> ELSTSLYKKAGFHHHHHHENLYFQDSNTKGWSEVLKGSECKPRPIVVPVSETHPELTSQRFNPPCVTLMRCGGCCNDESLECVPTEEVNVTMELLGAS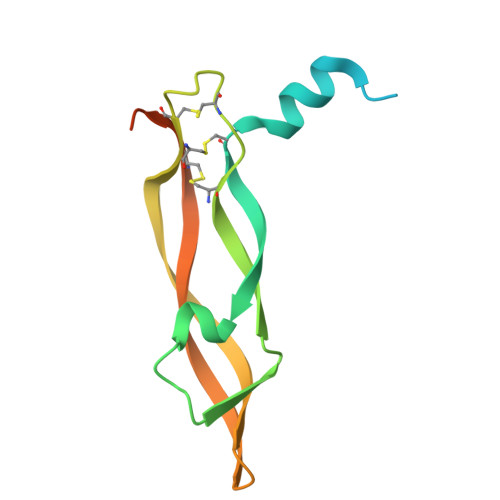GSGSNGMQRLSFVEHKKCDCRPRFTTTPPTTTRPPRRRR2-hydroxy-5-(thiophen-3-yl)benzoic acid | C11 H8 O3 S | 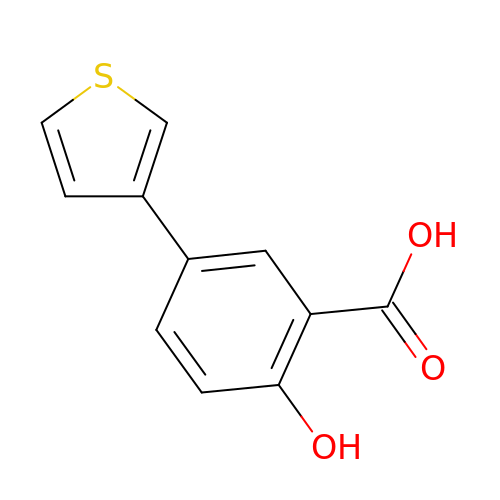ZGSXCSMJOZJLKM-UHFFFAOYSA-N> NTSLEAIVQNASSDNQGIQLSAVQAARKLLSSDRNPPIDDLIKSGILPILVHCLERDDNPSLQFEAAWALTNIASGTSEQTQAVVQSNAVPLFLRLLHSPHQNVCEQAVWALGNIIGDGPQCRDYVISLGVVKPLLSFISPSIPITFLRNVTWVMVNLCRHKDPPPPMETIQEILPALCVLIHHTDVNILVDTVWALSYLTDAGNEQIQMVIDSGIVPHLVPLLSHQEVKVQTAALRAVGNIVTGTDEQTQVVLNCDALSHFPALLTHPKEKINKEAVWFLSNITAGNQQQVQAVIDANLVPMIIHLLDKGDFGTQKEAAWAISNLTISGRKDQVAYLIQQNVIPPFCNLLTVKDAQVVQVVLDGLSNILKMAEDEAETIGNLIEECGGLEKIEQLQNHENEDIYK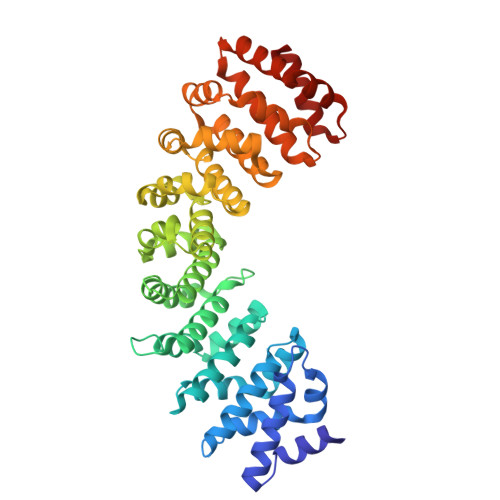LAYEIIDQFF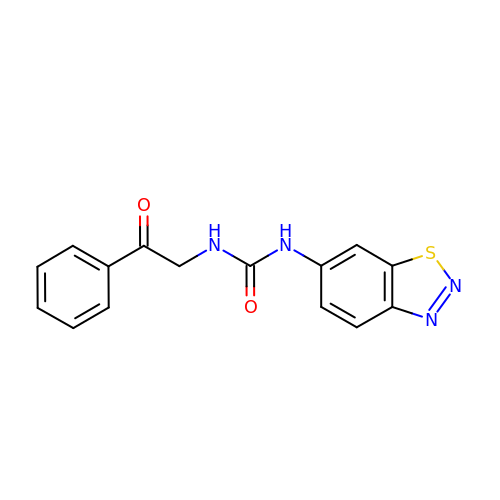1-(1,2,3-benzothiadiazol-6-yl)-3-(2-oxo-2-phenylethyl)urea | C15 H12 N4 O2 S | PKHSKYFMULMNOC-UHFFFAOYSA-N>[4x]MAEAGITGTWYNQLGSTFIVTAGADGALTGTYESAVGNAESRYVLTGRYDSAPATDGSGTALGWTVAWKNNYRNAHSATTWSGQYVGGAEARINTQWLLTSGTTEANA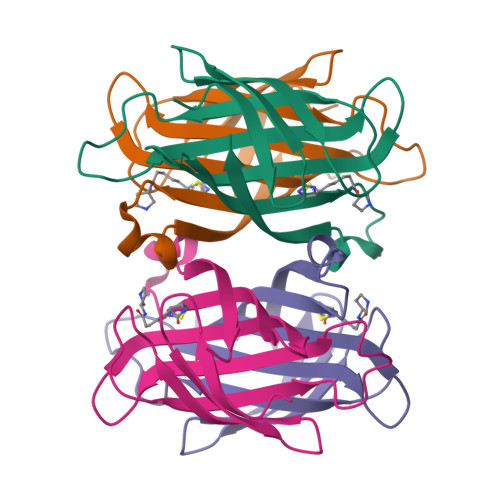WKSTLVGHDTFTKVKPSAAS>MKDLKGTKTAENLKQGFIGESMANRRYLYFAKRADEEGYPEIAGLLRSIAEGETAHAFGHLDFIRQGGLTDPATDKPIGTLEQMIESAIAGETYEWTQMYPGFAKVAREEGFPEVAEWFETLARAEK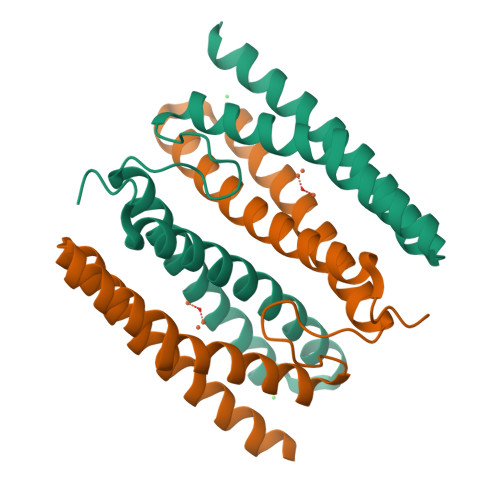SHAEKFQNVLKQLKGGT[2x]Phosphorylation of CTD residues is thought to recruit multiple co-factors, including the essential and conserved transcription factor Spt6, which directly binds to and co-localizes with RNAPII at sites of transcription. The C-terminal region (residues 1250–1440) comprises a tandem SH2 (tSH2) domain that is tethered to the core by a flexible 21-residue helix and contains both of the two known SH2 structural motifs in yeast. The N-terminal module (nSH2) resembles a canonical SH2 domain while the C-terminal module (cSH2) is vestigial and does not conserve the residues that are normally associated with binding to pY-containing peptides that comprise the vast majority of known SH2 domain ligands. We therefore took an unbiased approach to map the tSH2 domain binding site within RNAPII and, contrary to the earlier assumptions, found that Spt6 tSH2 directly binds the flexible, 86 residue Rpb1 linker (residues 1456–1541) that tethers the heptad CTD repeats to the RNAPII core.

To visualize the basis for this interaction, we determined a crystal structure of Spt6 tSH2 in complex with Rpb11468-1500 pT1471,pS1493 (multiple attempts to determine the structure of a complex with Rpb11468-1500 pY1473,pS1493 were unsuccessful). The unit cell and space group were the same as the earlier pS1493 complex crystal, and molecular replacement followed by refinement against 1.8 Å data to Rwork/Rfree values of 16.2%/19.8% revealed a very similar structure, with additional electron density corresponding to the N-terminal region of the Rpb1 peptide that includes pT1471. The unmodified Rpb1 Y1473 side chain occupies the typical position of the phenolic ring of pY, while the phosphate is instead contributed by pT. The phosphate is displaced 3–3.5 Å from the canonical location, and is hydrogen-bonded to the Y1473 hydroxyl via an ordered water molecule. This allows many of the interactions that stabilize binding in conventional SH2 domain interactions to be conserved in the Spt6-pT complex. For example, the water molecule that bridges the T1471 phosphate and the Y1473 hydroxyl is anchored to Spt6 through hydrogen bonds with the hydroxyl group and main chain nitrogen of S1285, which is analogous to the SH2 BC2 residue that in many SH2 domains is a serine or threonine that hydrogen bonds with the tyrosine phosphate. Similarly, Spt6 R1282 (SH2 βB5) hydrogen bonds the phosphate, as it does in canonical SH2-pY interactions. The 3–3.5 Å displacement of the phosphate relative to conventional pY complexes allows formation of an additional hydrogen bond interaction with the main chain carbonyl of Spt6 G1264 (SH2 αA2). In many SH2 domains, the αA2 residue is an arginine or lysine that forms a cation-pi interaction with the pY, so a glycine in this position may open the pocket to allow the displacement of the phosphate seen in our structure.

> GIDPFTAKRTHRVINHPYYFPFNGRQAEDYLRSKERGEFVIRQSSRGDDHLVITWKLDKDLFQHIDIQELEKENPLALGKVLIVDNQKYNDLDQIIVEYLQNKVRLLNEMTSSEKFKSGTKKDVVKFIEDYSRVNPNKSVYYFSLNHDNPGWFYLMFKINANSKLYTWNVKLTNTGYFLVNYNYPSVIQLCNGFKTLLKSNSSKNRMNNYR;> CGGVTPYSNESGLVNADLDVKDELMFSPLVDSGS In this work, we exhaustively probe the ability of all 36 immobile HJ sequences to form DNA crystals in two different designed systems. Three separate self-assembling DNA crystal systems are described in this report: the “4 × 5” and “4 × 6” designs (collectively referred to as the 4 × N systems), and a third construct with a “scrambled” sequence variant of the 4 × 6 lattices. Self-assembly was mediated by three constituent oligonucleotides: (S1) containing four sequence repeats of either 5 or 6 bases; (S2) composed of 21 bases containing complementary regions to both (S1); and (S3) which forms the second junction crossover. The HJ serves as the fundamental component at the core of each unit, and the ultimate assembly of the full lattice is facilitated by the complementary 2-base sticky ends that tail each duplex.

The 4 × 5 system robustly crystallized with 75% of the junctions, and we obtained crystals in all but 9 of 36 sequences. Pos1 and 2 were readily observable in the electron density maps at either one or both of these conserved sites in a significant number of the structures, with no apparent respect to motif or symmetry. However, in the majority of the crystal structures reported here, the cacodylate anion indeed fits best into the electron density map of our X-ray structures, due to the presence of sodium cacodylate in the crystallization solution.

> GAGCAGACCAG;> ACACCACTCA;> CTTGT;> TCTGAGTGGGGTCTGC>MNDQTQFTERALTILTLAQKLASDHQHPQLQPIHILAAFIETPEDGSVPYLQNLIEKGRYDYDLFKKVVNRNLVRIPQQQPAPAEITPSYALGKVLQDAAKIQKQQKDSFIAQDHILFALFNDSSIQQIFKEAQVDIEAIKQQALELRGNTRIDSRGADTNTPLEYLSKYAIDMTEQARQGKLDPVIGREEEIRSTIRVLARRIKSNPCLIGEPGIGKTAIIEGVAQRIIDDDVPTILQGAKLFSLDLAALTAGAKYKGDFEERFKGVLKEIEESKTLIVLFIDEIHMLMGNGKDDAANILKPALSRGQLKVIGATTNNEYRSIVEKDGAFERRFQKIEVAEPSVRQTVAILRGLQPKYEIHHGVRILDSALVTAAQLAKRYLPYRRLPDSALDLVDISCAGVAVARDSKPEELDSKERQLQLIQVEIKALERDEDADSTTKDRLKLARQKEASLQEELEPLRQRYNEEKHGHEELTQAKKKLDELENKALDAERRYDTATAADLRYFAIPDIKKQIEKLEDQVAEEERRAGANSMIQNVVDSDTISETAARLTGIPVKKLSESENEKLIHMERDLSSEVVGQMDAIKAVSNAVRLSRSGLANPRQPASFLFLGLSGSGKTELAKKVAGFLFNDEDMMIRVDCSELSEKYAVSKLLGTTAGYVGYDEGGFLTNQLQYKPYSVLLFDEVEKAHPDVLTVMLQMLDDGRITSGQGKTIDCSNCIVIMTSNLGAEFINSQQGSKIQESTKNLVMGAVRQHFRPEFLNRISSIVIFNKLSRKAIHKIVDIRL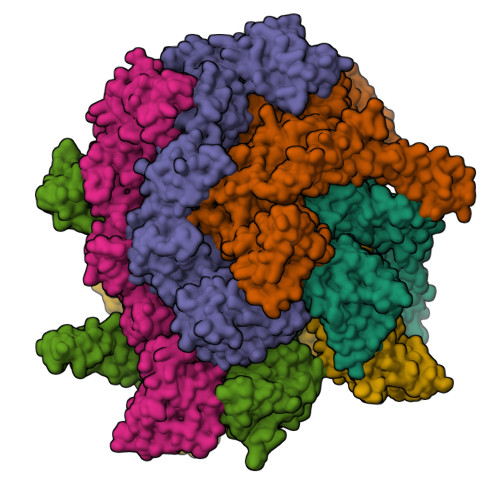KEIEERFEQNDKHYKLNLTQEAKDFLAKYGYSDDMGARPLNRLIQNEILNKLALRILKNEIKDKETVNVVLKKGKSRDENVPEEAEECLEVLPNHEATIGADTLGDDDNEDSMEIDDDLD[6x]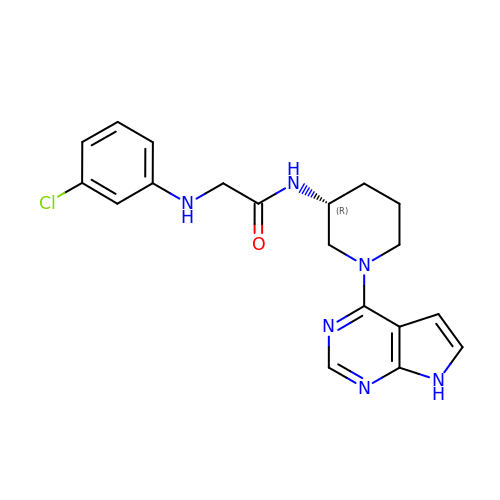N~2~-(3-chlorophenyl)-N-[(3R)-1-(7H-pyrrolo[2,3-d]pyrimidin-4-yl)piperidin-3-yl]glycinamide | C19 H21 Cl N6 O | SPSNKQVUYDXOGY-OAHLLOKOSA-N> LKALKKLA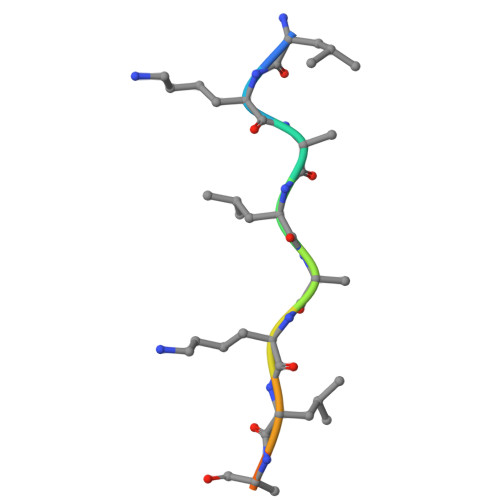KKY> MEQRSAETRIVEALLERRRLKDTDLVRARQLQAESGMGLLALLGRLGLVSERDHAETCAEVLGLPLVDARQLGDTPPEMLPEVQGLSLRFLKQFHLCPVGERDGRLDLWIADPYDDYAIDAVRLATGLPLLLHVGLRSE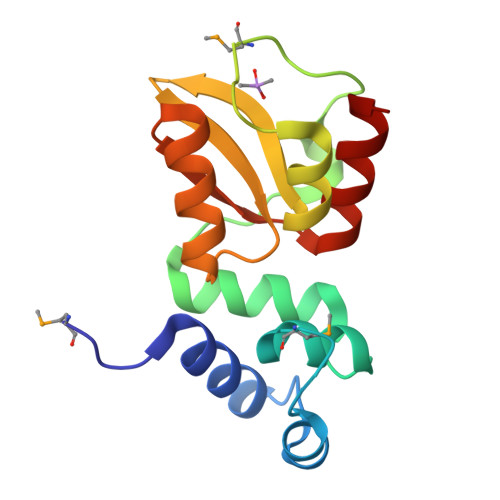IDDLIERWYG> UAGCUCC;>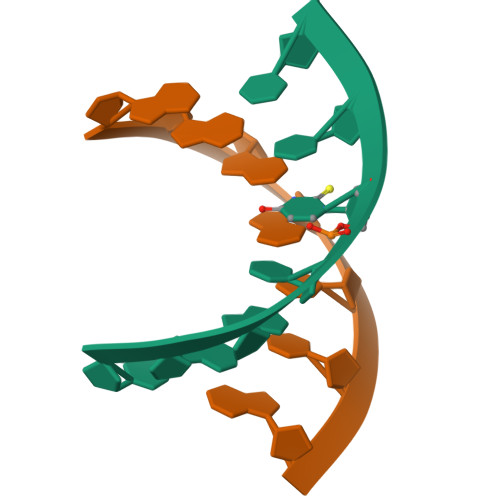 GGAGCUA>MVGGVVIA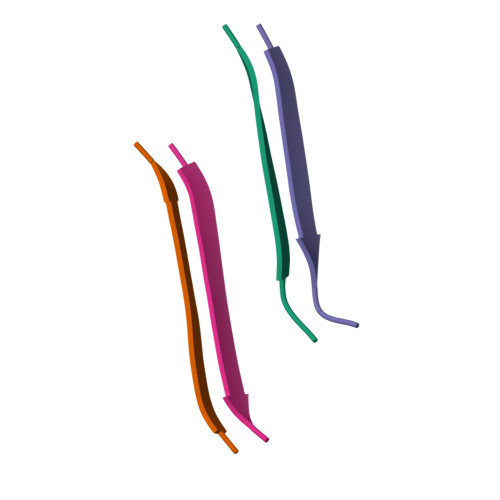[4x]>MEDPLIGRDSLGGGGTDRVRRSEAITHGTPFQKAAALVDLAEDGIGLPVEILDQSSFGESARYYFIFTRLDLIWSLNYFALLFLNFFEQPLWCEKNPKPSCKDRDYYYLGELPYLTNAESIIYEVITLAILLVHTFFPISYEGSRIFWTSRLNLVKVACVVILFVDVLVDFLYLSPLAFDFLPFRIAPYVRVIIFILSIRELRDTLVLLSGMLGTYLNILALWMLFLLFASWIAFVMFEATQQGLTVFTSYGATLYQMFILFTTSNNPDVWIPAYKSSRWSSVFFVLYVLIGVYFVTNLILAVVYDSFKEQLAKQVSGMDQMKRRMLEKAFGLIDSDKNGEIDKNQCIKLFEQLTNYRTLPKISKEEFGLIFDELDDTRDFKINKDEFADLCQAIALRFQKEEVPSLFEHFPQIYHSALSQQLRAFVRSPNFGYAISFILIINFIAVVVETTLAIEESSAQKPWQVAEFVFGWIYVLEMALKIYTYGFENYWREGANRFDFLVTWVIVIGETATFITPDENTFFSNGAWIRYLLLARMLRLIRLLMNVQRYRAFIATFITLIPSLMPYLGTIFCVLCIYCSIGVQVFGGLVNAGNKKLFETELAEDDYLLFNFNDYPNGMVTLFNLLVMGNWQVWMESYKDLTGTWWSITYFVSFYVITILLLLNLVVAFVLEAFFTELDLEEEEKCQGQDSQE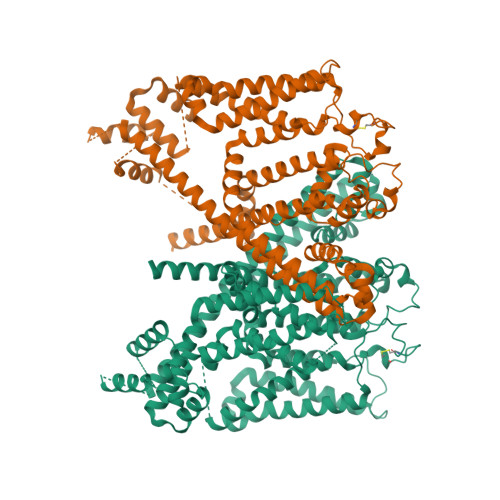KRNRRRSAGSKSRSQRVDTLLHHMLGDELSKPECSTSDT[2x]> MFKAQATFSRYSAAVSLLLLFSGAAQAAPQSITTLPLQPDGENRWRLPAGEYQGQFTIEQPMQLRCEPGAVIQSQGQGSSLLISAPDVLVEGCTLYEWGSDLTAMDSAVFILPAAERAQISN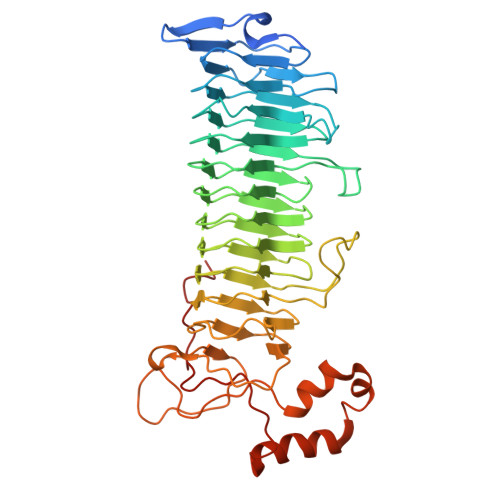NRMRGPGFGVFVDGTRDVQVIGNEIDGDAGVRSQDRGNGIHLFAVSGARVLHNHVRNARDGIYIDTSNGNHLEGNVIEDVRYGVHYMFANENSLIDNVTRRTRTGYALMQSRKLTVTGNRSEQDQNYGILMNYITYSTITGNFVSDVQRGDTGGDSMISGGEGKALFIYNSLFNTIENNHFEKSSLGIHLTAGSEDNRISGNAFVGNQQQVKYVASRTQEWSVDGRGNYWSDYLGWDRNNDGLGDIAYEPNDNVDRLLWLYPQVRLLMNSPSIEVLRWVQRAFPVIKSPGVQDSHPLMKLPTEKLLTEKQEPTS> LRSTGVSLYYRATAELDRLRGMLRGRARLERKV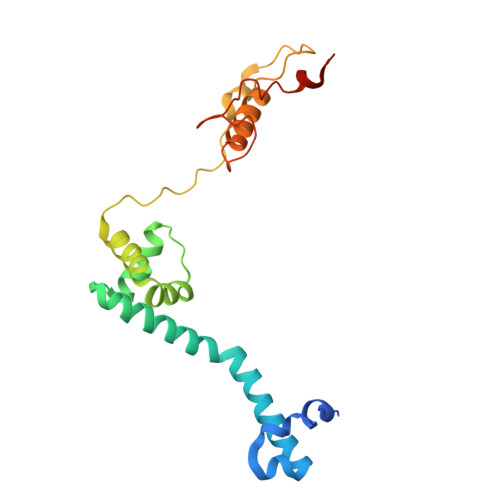GLKRITFLMRTQTRYRVEQKAHWERAIVRKNVDSAAHEHGSGWQHLRNDLARQNLMLLPRTQQQLAQYEPLAFRAVMELCASRVAPPPPPMTAQVPEEAYATRPEDPKVAHPAARRQLEECVERMLCTGRSDVLQREGPRTTQAWMDAWKEYDLGSAAQK>MDFSKLPKIRDEDKESTFGYVHGVSGPVVTACDMAGAAMYELVRVGHSELVGEIIRLEGDMATIQVYEETSGVSVGDPVLRTGKPLSVELGPGIMGAIFDGIQRPLSDISSQTQSIYIPRGVNVSALSRDIKWEFIPSKNLRVGSHITGGDIYGIVNENSLIKHKIMLPPRSRGSVTYIAPPGNYDASDVVLELEFEGVKEKLSMVQVWPVRQVRPVTEKLPANHPLLTGQRVLDALFPCVQGGTTAIPGAFGCGKTVISQSLSKYSNSDVIIYVGCGERGNEMSEVLRDFPELTMEVDGKVESIMKRTALVANTSNMPVAAREASIYTGITLSEYFRDMGYHVSMMADSTSRWAEALREISGRLAEMPADSGYPAYLGARLASFYERAGRVKCLGNPEREGSVSIVGAVSPPGGDFSDPVTSATLGIVQVFWGLDKKLAQRKHFPSVNWLISYSKYMRALDEYYDKHFTEFVPLRTKAKEILQEEEDLAEIVQLVGKASLAETDKITLEVAKLIKDDFLQQNGYTPYDRFCPFYKTVGMLSNMISFYDMARRAVETTAQSDNKITWSIIREHMGEILYKLSSMKFKDPVKDGEAKIKADYAQLLEDMQNAFRSLED[3x];>MALRAMRGIVNGAAPELPVPTGGPMAGAREQALAVSRNYLSQPRLTYKTVSGVNGPLVILDHVKFPRYAEIVHLTLPDGTKRSGQVLEVSGSKAVVQVFEGTSGIDAKKTSCEFTGDILRTPVSEDMLGRVFNGSGKPIDRGPVVLAEDFLDIMGQPINPQCRIYPEEMIQTGISAIDGMNSIARGQKIPIFSAAGLPHNEIAAQICRQAGLVKKSKDVVDYSEENFAIVFAAMGVNMETARFFKSDFEENGSMDNVCLFLNLANDPTIERIITPRLALTTAEFLAYQCEKHVLVILTDMSSYAEALREVSAAREEVPGRRGFPGYMYTDL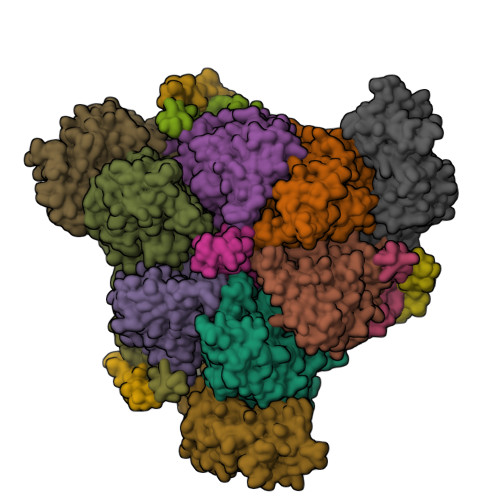ATIYERAGRVEGRNGSITQIPILTMPNDDITHPIPDLTGYITEGQIYVDRQLHNRQIYPPINVLPSLSRLMKSAIGEGMTRKDHADVSNQLYACYAIGKDVQAMKAVVGEEALTSDDLLYLEFLQKFEKNFITQGPYENRTVYETLDIGWQLLRIFPKEMLKRIPQSTLSEFYPRDSAKH[3x];> MSGKDRIEIFPSRMAQTIMKARLKGAQTGRNLLKKKSDALTLRFRQILKKIIETKMLMGEVMREAAFSLAEAKFTAGDFSTTVIQNVNKAQVKIRAKKDNVAGVTLPVFEHYHEGTDSYELTGLARGGEQLAKLKRNYAKAVELLVELASLQTSFVTLDEAIKITNRRVNAIEHVIIPRIERTLAYIITELDEREREEFYRLKKIQEKKKIIKEKSEKDLERRRAAGEVMEPANLLAEEKDEDLLFE;>MALSDADVQKQIKHMMAFIEQEANEKAEEIDAKAEEEFNIEKGRLVQTQRLKIMEYYEKKEKQIEQQKKIQMSNLMNQARLKVLRARDDLITDLLNEAKQRLSKVVKDTTRYQVLLDGLVLQGLYQLLEPRMIVRCRKQDFPLVKAAVQKAIPMYKIATKKDVDVQIDLEAYLPEDIAGGVEIYNGDRKIKVSNTLESRLDLIAQQMMPEVRGALFGANANRKFLD[3x];>[3x]MASQSQGIQQLLQAEKRAAEKVADARKRKARRLKQAKEEAQMEVEQYRREREQEFQSKQQAAMGSQGNLSAEVEQATRRQVQGMQSSQQRNRERVLTQLLGMVCDVRPQVHPNYRITV;>[3x]GMSFIKVGIKMGGLTSEQYHSQVVGKIGYIARCMQTIDPENNLKKIREDYQDVLIWAEKNYRFEEILEASKSGKCPNDLDALSRRSLILQELLRLVSSISPFKMKLDLIESQYEKMKQHVNLWKSDYHVKLNQLNQLTDYLKNAAPTPKNNFLRAMTSVLQMQIAQYGITEDNEGINQLFKLGLHLLAMANEKIDEQYHLFKGYVKDQPEESPFEGILPAEDQKILVKTMIDYAMPKLSSKVLQDKLSALSSSDVLTKTLLDSIDRIVKENEKLNALSKDYKDHDGDYKDHDIDYKDDDDK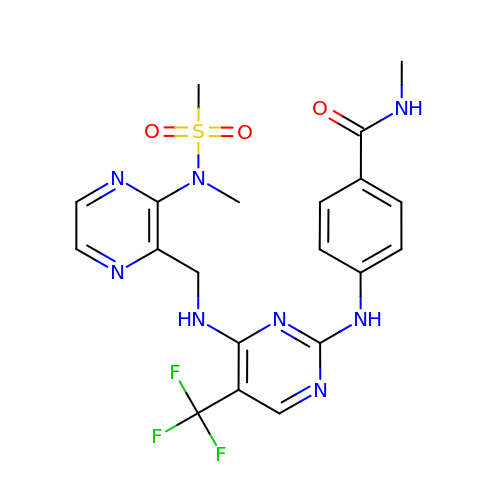~{N}-methyl-4-[[4-[[3-[methyl(methylsulfonyl)amino]pyrazin-2-yl]methylamino]-5-(trifluoromethyl)pyrimidin-2-yl]amino]benzamide | C20 H21 F3 N8 O3 S | FWLMVFUGMHIOAA-UHFFFAOYSA-N> MGKLIRLELFNFKSYKGHHTLLFGDSYFTSIIGPNGSGKSNSMDAISFVLGIKSSHLRSSNLRDLIYRGRVMKTSKIQDDGTTAPATNGDVNGYENGDAGDDEDTSQRTSRNDPKTAWVMAVYEDDAGELHRWKRTITANGTSEYRINDRVVNAQQYNEALEKENILIKARNFLVFQGDVEAIASQSPQDLTRLIEQISGSLEYKEEYERLEEEVRQATEEQAYKLQRRRAANSEIKQYMEQ;> MASKAIVQMAKILRKELSEEKEVIFTDVLKSQANTEPENITKREASRGFFDILSLATEGCIGLSQTEAFGNIKIDAKPALFERFI;> MAYIKRVIIKGFKTYRNETIIDNFSPHQNV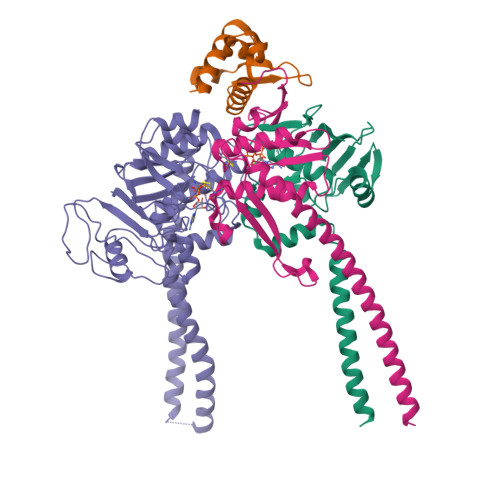IIGSNGSGKSNFFAAIRFVLSDDYSNLKREERQGLIHQGSGGSVMSASVEIVFHDPDHSMILPSGVLSRGDDEVTIRRTVGLKKDDYQLNDRNVTKGDIVRMLETAGFSMNNPYNIVPQGKIVALTNAKDKERLQLLEDVVGAKSFEVKLKASLKKMEETEQKKIQINKEMGELNSKLSEMEQERKELEKYNELERNRKIYQFTLYDRELNEVINQMERLDGDYNNTVYSSESSKHPTSLVPRGSDITSDQLLQRLNDMNTEISGLKNVNKRAFENFKKFNERRKDLAERASELDESKDSIQDLIVKLKQQKVNAVDSTFQKVSENFEAVFERLVPRGTAKLIIHRKNDNANDHDESIDVDMDAESNESQNGKDSEIMYTGVSISVSFNSKQNEQLHVEQLSGGQKTVCAIALILAIQMVDPASFYLFDEIDACLDKQYRTAVATLLKELSKNAQFICTTFRTDMLQVADKFFRVKYECKISTVIEVNREEAIGFIRGSNKFAEV;> MVTENPQRLTVLRLATNKGPLAQIWLASNMSNIPRGSVIQTHIAESAKEIAKASGSDDESGDNEYITLRTSGELLQGIVRVYSKQATFLLTDIKDTLTKISMLFKTSQKMTSTVNRLNTVTRVHQLMLEDAVTEREVLVTPGLEFLDDTTIPVGLMAQENPNLRAMDRLDHVRKQLEQTEQEFEASKAKLRQARESFQAVKQKRLELFNKAFTHIQEQITHVYKELTRSEAYPLGGQAYLDIEEDTDTPFLSGVKYHAMPPCKRFRDMEHLSGGEKTMAALALLFAIHSYQPSPFFVLDEVDCALDNANVEKIKKYIREHAGPGMQFIVISLKPALFQASESLIGVYRDQEANTSRTLTLDLRKYRHHHHHH The mtrR gene encodes a transcriptional repressor of the mtrCDE multidrug efflux transporter genes. Previously, we showed that MtrR adopts a typical TFR fold: MtrR is a functional homodimer composed of nine α-helices that form a C-terminal ligand-binding/dimerization domain and an N-terminal helix-turn-helix (HTH) DNA-binding motif. For example, MtrR represses directly the expression of rpoH, an essential alternate sigma factor that is important for gonococcal oxidative stress responses; DNase protection assays revealed direct MtrR binding to the rpoH operator. In this work, we report the crystal structures of MtrR bound to the mtrCDE and rpoH operators, which reveal a conserved, but degenerate, DNA consensus binding site 5′-MCRTRCRN4YGYAYGK-3′.

MtrR was crystallized with a 21-basepair oligoduplex of the rpoH operator. The crystal structure of MtrR-rpoH complex was determined to 2.80 Å resolution by molecular replacement in combination with single-wavelength anomalous dispersion (MR-SAD) methods using Semet-MtrR. This structure was then used to solve the structure of a higher resolution Semet-MtrR-rpoH complex to 2.60 Å resolution by molecular replacement (MR) resulting in final Rwork and Rfree values of 19.9% and 25.6%, respectively, after refinement and model rebuilding. The asymmetric unit of the MtrR-rpoH operator complex crystal structure contains a functional homodimer of MtrR bound to the double-stranded 21-mer encompassing the rpoH operator site. The root mean square deviation (RMSD) of the pairwise alignments of all corresponding Cα atoms of the two subunits in the asymmetric unit is 0.11 Å. Furthermore, the MtrR residues that contact the rpoH DNA are the same for each subunit. However, the average major groove width is 12.5 Å compared to the average major groove width of 11.4 Å for ideal B-DNA. Therefore, the major grooves of the DNA are slightly widened, which likely occurs upon formation of the complex when α3 and α3′ insert into adjacent major grooves of the DNA. ; however, in the MtrR-rpoH operator structure, one subunit recognizes a 5′-TpG-3′ step at position 13Bp14B and the other recognizes a 5′-CpG-3′ step at position 14Ap15A, again where stacking between the R44 side chain and cytidine is maintained. Intriguingly, we observed nearly a ∼6-fold higher affinity of MtrR for rpoH than mtrCDE. Indeed, comparing the contacts of MtrR to the pyrimidine in the 5′-YpA-3′ steps within the rpoH and mtrCDE operators reveals shorter distances between these interactions in the MtrR-rpoH operator complex.

>[2x]SNAMRKTKTEALKTKEHLMLAALETFYRKGIARTSLNEIAQAAGVTRGALYWHFKNKEDLFDALFQRICDDIENCIAQDAADAEGGSWTVFRHTLLHFFERLQSNDIHYKFHNILFLKCEHTEQNAAVIAIARKHQAIWREKITAVLTEAVENQDLADDLDKETAVIFIKSTLDGLIWRWFSSGESFDLGKTAPRIIGIMMDNLENHPCLRRK>[2x]KNNPDPTIYPVLDWNDIKFQDVIGEGNFGQVLKARIKKDGLRMDAAIKRMKEYASKDDHRDFAGELEVLCKLGHHPNIINLLGACEHRGYLYLAIEYAPHGNLLDFLRKSRVLETDPAFAIANSTASTLSSQQLLHFAADVA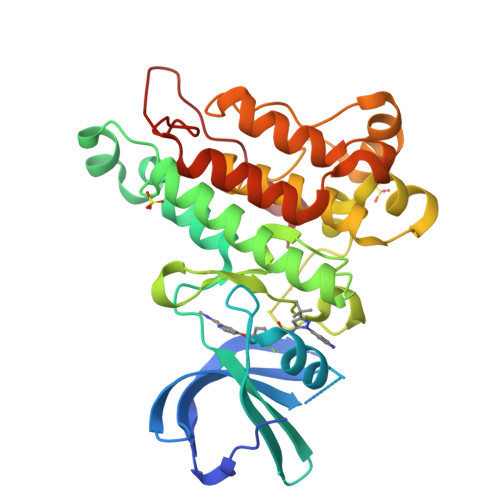RGMDYLSQKQFIHRDLAARNILVGENYVAKIADFGLSRGQEVYVKKTMGRLPVRWMAIESLNYSVYTTNSDVWSYGVLLWEIVSLGGTPYCGMTCAELYEKLPQGYRLEKPLNCDDEVYDLMRQCWREKPYERPSFAQILVSLNRMLEERKTYVNTTLYEKFTYAGIDCSAEEAA> MTHAGMKASLPNRVMLNAYPDSIDGDLAGTVRMLQRPEFTDAFGLFYVLPSIFNSDLDRGFSIIDYDLNSDLASAEDLAALDELGIMLKFDMVLNHLSVGSPQFQDLL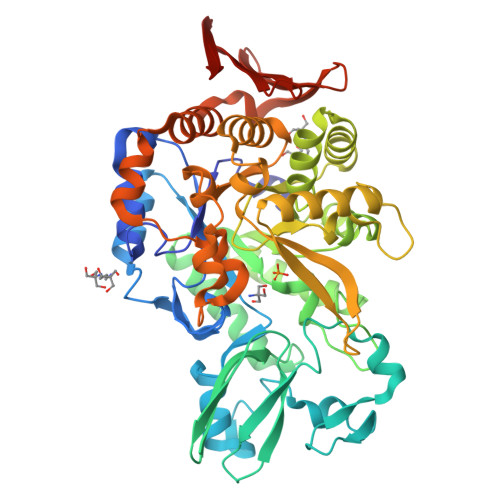KHGDDSAFRDFFIDWNEFWEGEGELHADGHVVPSPEHLDRLFMRKPGLPILQVRFPDGSDRFYWNTFYQRVETIDGERSYLGQMDLNAESPRVWTFYRETFEKLARYGAKIVRLDAFAYLHKAVGDTNFFNTPGTWDHLDRLRTISEENGLVLLPEIHGEYGTKIHEELSDRDYPVYDFFFPGLVIDAIDSASNTHLLRWIDEIIERDIATVNMLGCHDGIPVIDLKGGPTGQGLLPDATIEAMISRLLERGGRVKNLYGADGTKVSYYQVNATFFSALGESDARLRLARAIQLFVPGTPQVWYLDLFAGANDVEAADRAGADGHKEINRTNLSAADVEAGLARPIVLDQLEMIRLRNASPAFDGRFEVVPTDDTRLQLRWQNGSTVALLDADLATERFTITHEHDGHTEILGYDLEHHHHHH H. pylori adhesin A (HpaA) stands out as a pivotal adhesin that plays an indispensable role in the successful establishment of colonization by the pathogen. Originally characterized as a neuraminyllactose-binding hemagglutinin, HpaA is a 26 kDa lipoprotein found on the bacterial surface and flagellar sheath. The gene encoding HpaA is prevalent in most H. pylori strains, and its amino-acid sequence displays a high degree of conservation among H. pylori isolates. For these reasons, HpaA is considered a promising vaccine candidate against H. pylori.

The crystal structure of HpaA26–233 was determined using a C-terminally his-tagged protein construct, excluding the first 25 amino acids from the mature lipoprotein. Initial attempt to crystallize the full-length HpaA2-233 was unsuccessful, leading to the engineering of the HpaA26–233 construct resolved at 2.9 Å resolution. The protein crystallized as two homodimers within the asymmetric unit of the P21 space group, a conformation that likely results from the large crystal lattice and tight packing of the protein within the crystal, with 40% solvent. Further characterization of the molecule using multi-angle light scattering confirmed that HpaA26-233 exists as a homogeneous and monomeric species in solution, with a calculated molecular mass of 22.5 kDa. The crystal structure reveals that HpaA is an elongated protein consisting of two successive antiparallel β-sheets, with an apical extension protruding from a more globular domain composed of one of the β-sheets surrounded by three α-helices (α1-α3-α4) stabilized together by hydrophobic interactions. The overall fold is well conserved among the three homologs, except for the apical domain, which exhibits significant structural and sequence variations. Of particular interest, the apical loop L5 harbors an intriguing feature in the form of a hydrophobic 118-LLF-120 motif that is fully exposed to the aqueous environment. Consistently, all four 118-LLF-120 motifs observed in the asymmetric unit are engaged in similar crystal contacts with adjacent HpaA molecules, burying the leucine and phenylalanine residues within a neighboring cavity formed between the α-helices α1 and α3. According to the cell adhesion assays, the flow cytometric analysis unveils the significant contribution of the 118-LLF-120 apical loop L5 to host-cell recognition, as mutation within this loop resulted in a 55% decrease in binding association with AGS cells. Interactions mediated by this motif were severely impeded by reverse charge mutations (107-EETIQEE-113 mutants) leading to a substantial loss of binding activity with a 50% decrease observed.

>[4x]MALDEKILLLRPAFQYSDNIAKEYENKFKNQTALKVEQILQNQGYKVISVDSSDKDDLSFSQKKEGYLAVAMNGEIVLRPDPKRTIQKKSEPGLLFSTGLDKMEGVLIPAGFVKVTILEPMSGESLDSFTMDLSELDIQEKFLKTTHSSHSGGLVSTMVKGTDNSNDAIKSALNKIFANIMQEIDKKLTQKNLESYQKDAKELKGKRNRHHHHHH>[2x]GGDPHMMFGKKKNNGGSSTARYSAGNKYNTLSNNYALSAQQLLNASKIDDIDSMMGFERYVPPQYNGRFDAKDIDQIPGRVGWLTNMHATLVSQETLSSGSNGGGNSNDGERVTTNQGISGVDFYFLDEEGGSFKSTVVYDPYFFIACNDESRVNDVEELVKKYLESCLKSLQIIRKEDLTMDNHLLGLQKTLIKLSFVNSNQLFEARKLLRPILQDNANNNVQRNIYNVAANGSEKVDAKHLIEDIREYDVPYHVRVSIDKDIRVGKWYKVTQQGFIEDTRKIAFADPVVMAFDIETTKPPLKFPDSAVDQIMMISYMIDGEGFLITNREIISEDIEDFEYTPKPEYPGFFTIFNENDEVALLQRFFEHIRDVRPTVISTFNGDFFDWPFIHNRSKIHGLDMFDEIGFAPDAEGEYKSSYCSHMDCFRWVKRDSYLPQGSQGLKAVTQSKLGYNPIELDPELMTPYAFEKPQHLSEYSVSDAVATYYLYMKYVHPFIFSLCTIIPLNPDETLRKGTGTLCEMLLMVQAYQHNILLPNKHTDPIERFYDGHLLESETYVGGHVESLEAGVFRSDLKNEFKIDPSAIDELLQELPEALKFSVEVENKSSVDKVTNFEEIKNQITQKLLELKENNIRNELPLIYHVDVASGYPNIMTTNRLQPDSIKAERDCASCDFNRPGKTCARKLKWAWRGEFFPSKMDEYNMIKRALQNETFPNKNKFSKKKVLTFDELSYADQVIHIKKRLTEYSRKVYHRVKVSEIVEREAIVCQRENPFYVDTVKSFRDRRYEFKGLAKTWKGNLSKIDPSDKHARDEAKKMIVLYDSLQLAHKVILNSFYGYVMRKGSRWYSMEMAGITCLTGATIIQMARALVERVGRPLELDTDGIWCILPKSFPETYFFTLENGKKLYLSYPCSMLNYRVHQKFTNHQYQELKDPLNYIYETHSENTIFFEVDGPYKAMILPSSKEEGKGIKKRYAVFNEDGSLAELKGFELKRRGELQLIKNFQSDIFKVFLEGDTLEGCYSAVASVCNRWLDVLDSHGLMLEDEDLVSLICENRSMSKTLKEYEGQKSTSITTARRLGDFLGEDMVKDKGLQCKYIISSKPFNAPVTERAIPVAIFSADIPIKRSFLRRWTLDPSLEDLDIRTIIDWGYYRERLGSAIQKIITIPAALQGVSNPVPRVEHPDWLKRKIAT

At the eukaryotic replication fork, the family B replicative DNA polymerases epsilon (Pol ε) and delta (Pol δ) synthesize the leading and lagging strand, respectively. The exonuclease domains of family B polymerases have several highly-conserved motifs (named Exo-motifs), which include the catalytic residues (D290, E292, D383 and D477 in yeast Pol ε). The catalytic residues serve as ligands for two metal ions, and substituting both D290 and E292 with alanine abolishes the proofreading function of the polymerase, which in turn increases the in vitro mutation rate by ~100-fold. At present, many structures of family B DNA polymerases with proofreading capacity have been determined, and their overall structures are well conserved, consisting of a thumb, palm, fingers and the exonuclease domain.

The catalytic site of the exonuclease domain is supposed to harbor two metal ions, which are essential for the exonuclease activity. The published Pol ε wild-type exonuclease domain structure, solved by Jain et al., only possesses one metal ion, located at the B-site. Within another project we solved a Pol2CORE structure of a polymerase active site mutant, Pol2CORE M644G, which has an unaffected wild-type exonuclease domain. This structure of the wild-type exonuclease domain, solved at 2.5 Å resolution, contained two Ca2+ ions located at the A- and B-site of the exonuclease site. We used this structure to assess the impact of P301R substitution on the exonuclease domain and will refer to it as wild type for the purpose of exonuclease domain comparison.> MKRPVIILLLGIVTMCAMAQTGDKPVDLKEITSGMFYARSAGRGIRSMPDGEHYTEMNRERTAIVRYNYASGKAVDTLFSIERARECPFKQIQNYEVSSTGHHILLFTDMESIYRHSYRAAVYDYDVRRNLVKPLSEHVGKVMIPTFSPDGRMVAFVRDNNIFIKKFDFDTEVQVTT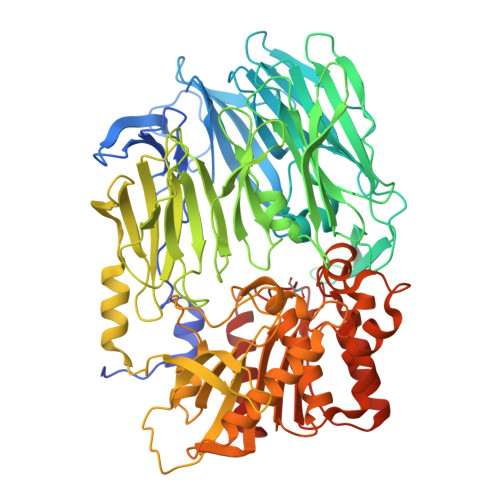DGQINSVLNGATDWVYEEEFGVTNLMSWSADNAFLAFVRSDESAVPEYRMPMYEDKLYPEDYTYKYPKAGEKNSTVSLHLYNVADRNTKSVSLPIDADGYIPRIAFTDNADELAVMTLNRLQNDFKMYYVHPKSLVPKLILQDMNKRYVDSDWIQALKFTAGGGFAYVSEKDGFAHIYLYDNKGVMHRRITSGNWDVTKLYGVDASGTVFYQSAEESPIRRAVYAIDAKGRKTKLSLNVGTNDALFSGNYAYYINTYSSAATPTVVSVFRSKGAKELRTLEDNVALRERLKAYRYNPKEFTIIKTQSALELNAWIVKPIDFDPSRHYPVLMVQYSGPNSQQVLDRYSFDWEHYLASKGYVVACVDGRGTGARGEEWRKCTYMQLGVFESDDQIAAATAIGQLPYVDAARIGIWGWSYGGYTTLMSLCRGNGTFKAGIAVAPVADWRFYDSVYTERFMRTPKENASGYKMSSALDVASQLQGNLLIVSGSADDNVHLQNTMLFTEALVQANIPFDMAIYMDKNHSIYGGNTRYHLYTRKAKFLFDNL>TLLGTALRPAATRVMLLGSGELGKEVAIECQRL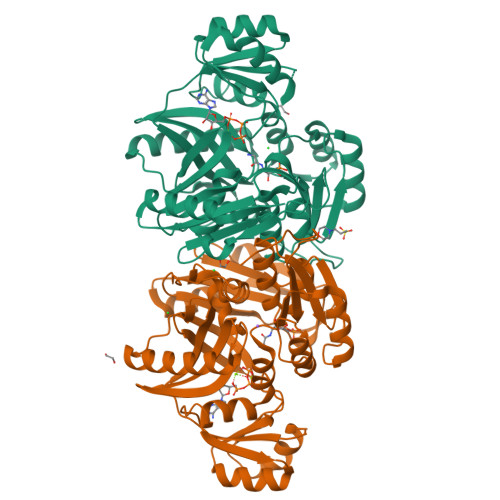GVEVIAVDRYADAPAMHVAHRSHVINMLDGDALRRVVELEKPHYIVPEIEAIATDMLIQLEEEGLNVVPCARATKLTMNREGIRRLAAEELQLPTSTYRFADSESLFREAVADIGYPCIVKPVMSSSGKGQTFIRSAEQLAQAWKYAQQGGRAGAGRVIVEGVVKFDFEITLLTVSAVDGVHFCAPVGHRQEDGDYRESWQPQQMSPLALERAQEIARKVVLALGGYGLFGVELFVCGDEVIFSEVSPRPHDTGMVTLISQDLSEFALHVRAFLGLPVGGIRQYGPAASAVILPQLTSQNVTFDNVQNAVGADLQIRLFGKPEIDGSRRLGVALATAESVVDAIERAKHAAGQVKVQG[2x]> MASNYNSGLKIGAWVGTQPSESAIKSFQELQGRKLDIVHQFINWSTDFSWVRPYADAVYNNGSILMITWEPWEYNTVDIKNGKADAYITRMAQDMKAYGKEIWLRPLHEANGDWYPWAIGYSSRVNTNETYIAAFRHIVDIFRANGATNVKWVFNVNCDNVGNGTSYLGHYPGDNYVDYTSIDGYNWGTTQSWGSQWQSFDQVFSRAYQALASINKPIIIAEFASAEIGGNKARWITEAYNSIR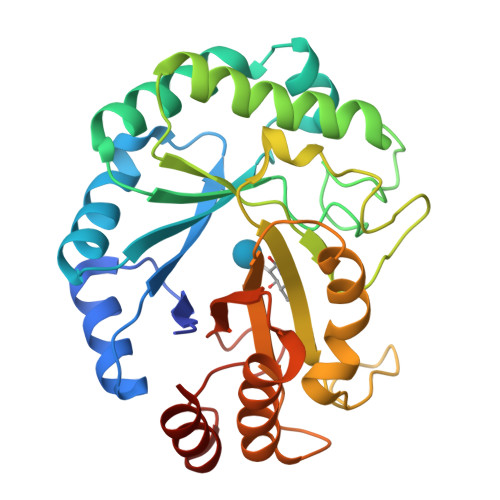TSYNKVIAAVWFHENKETDWRINSSPEALAAYREAIGAG> SFH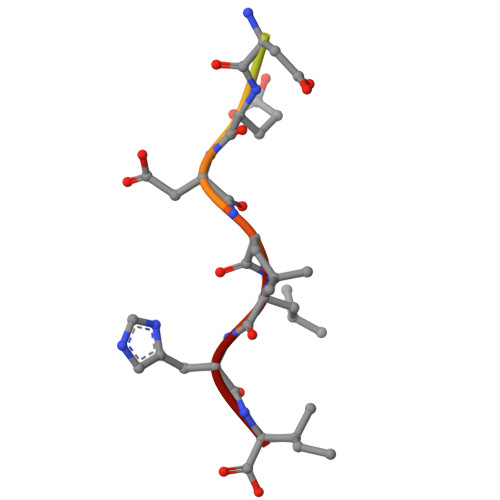DDSDEDLLHI> PVVIKTEGPAWTPLEPKLITRLADTVRTKGLRSPITMAEVEALMSSPLL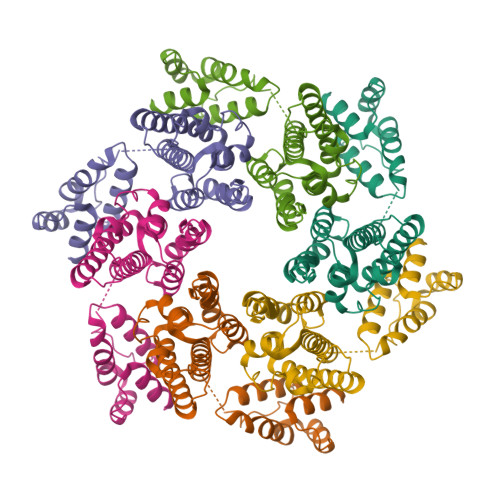PHDVTNLMRVILGPAPYALWMDAWGVQLQTVIAAATRDPRHPANGQGRGERTNLNRLKGLADGMVGNPQGQAALLRPGELVAITASALQAFREVARLAEPAGPWADIMQGPSESFVDFANRLIKAVEGSDLPPSARAPVIIDCFRQKSQPDIQQLIRTAPSTLTTPGEIIKYVLDRQ>[4x]AQCSVDIQGNDQMQFNTNAITVDKSCKQFTVNLSHPGNLPKNVMGHNWVLSTAADMQGVVTDGMASGLDKDYLKPDDSRVIAQTKLIGSGEKDSV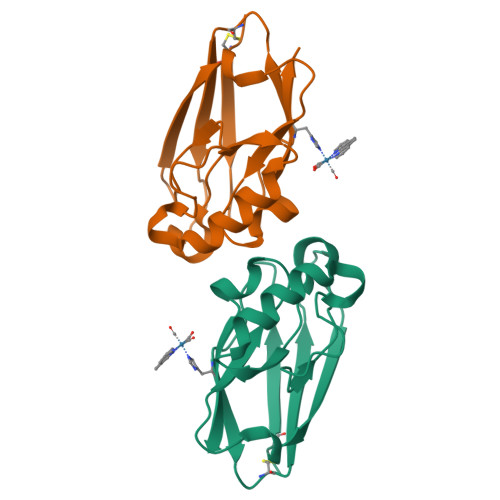TFDVSKLKEGEQYMFFCTFPGHSALMKGHLTLK>[2x]VNFPNIP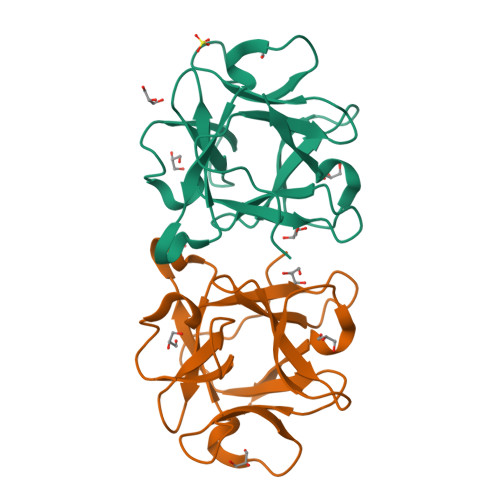AEGVQFRLRARDTGYVIYSRTENPPLVWQYNGPPYDDQLFTLIYGTGPRKNLYAIKSVPNGRVLFSRTSASPYVGNIAGDGTYNDNWFQFIQDDNDPNSFRIYNLASDTVLYSRTTADPKFGNFTGAKYDDQLWHFELV> SSNYCNQMMKSRNLTKDRCKPVNTFVHESLADVQAVCSQKNVACKNGQTNCYQSYSTMSITDCRETGSSKYPNCAYKTTQANKHIIVACEGN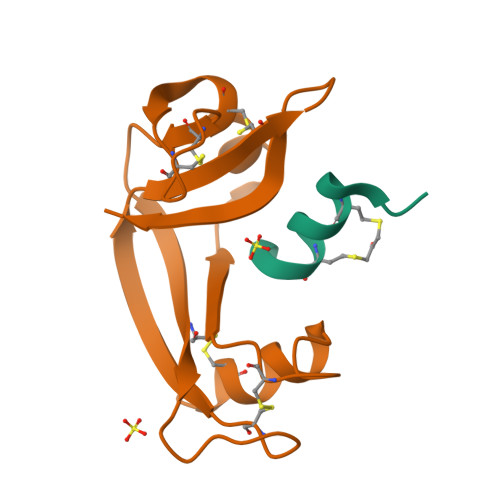PYVPVHFDASV;> XKETAAXKFEXQHMDS>[7x]MSLALSQIEIQQFLSEAHAEFQSEGFLLQGAVRTKSGTKGSIVHFPVFGEGMANQKAPQDDITPMNVSNRDAEAVIEDWYASEYADRSFQNKLAVNAVEEYAKLCAWAIGRRADQINIDTIAGATYSATPNDQQGALVPVGTTGFTFEKLRQAHRWLRQRSANRGKRTVIIDAIAEEQLLNVEQLTNSFYVNQKILDNDGLHGMTFLGMNFIVIPSMQEGGLPTTGGGTVGRAFFINEMAVGYAQSERLGGDISWENIKTSYLINMWMEAGAVVIDPKGLVEVDYLLEP;>MAFGINYMGRVSTSANNDTQKVWIYNGTATGSNETVATIAASGYFNAFMVNVALGKGPLGVG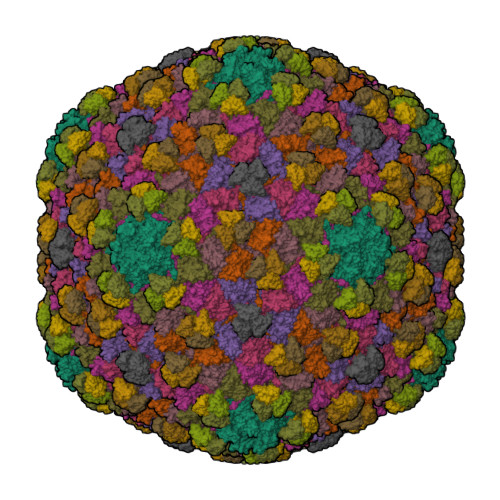DLIIINGNDASAFYTVQTITPNVTVSVFAASGVVGTSNIQDGAVTANKLATDSVTTVKILDDNVTSDKIAASVLKYVAVPLTAANIIAMNGAPVQVLAAGGANTVHLVEHACLMMTYGTTQFTGGGAIGLQYGNTAALAGEAASSTIAAANVQGAASTMDMVEGALSSGAFTAVANLGLFISNNTAAFAAGDSDFVLHLWYRTVPTV[7x]>MKLKSFGVFGNPIKHSKSPLIHNACFLTFQKKLGFLGHYRPILLPLESHIKNEFLHLGLSGANVTLPFKERAFQVCDKIKGIALECASINTLVLENDELVGYNTDALGFYLSLKHQNYQNALILGSGGSAKALACGLKKQGLKVSVLNRSPRGLDFFQRLGCDCFMEPPKSAFDLIINATSASLNNELPLNK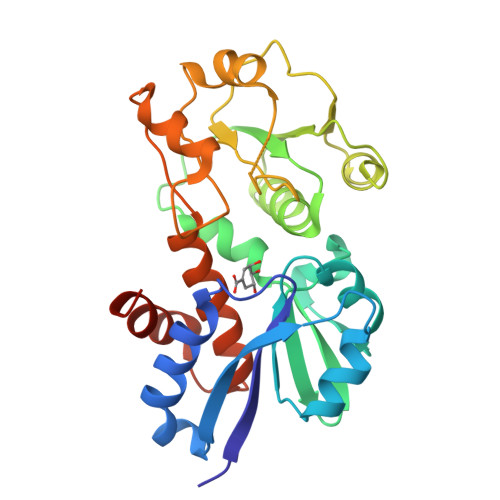EVLKGYFKEAKLAYDLAYGFLTPFLALAKELKIPFQDGKDMLIYQASLSFEKFSASQIPYSKAFEVMRSVFLEHHHHHH[2x]> MAVFADLDLRAGSDLKALRGLVETAAHLGYSVVAINHIVDFKEKKQEIEKPVAVSELFTTLPIVQGKSRPIKILTRLTIIVSDPSHCNVLRATSSRARLYDVVAVFPKTEKLFHIACTHLDVDLVCITVTEKLPFYFKRPPINVAIDRGLAFELVYSPAIKDSTMRRYTISSALNLMQICKGKNVIISSAAERPLEIRGPY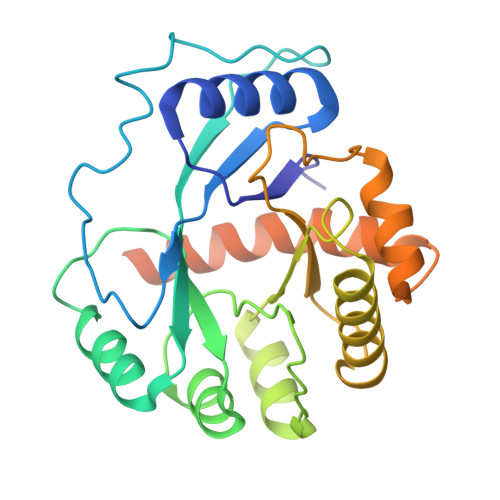DVANLGLLFGLSESDAKAAVSTNCRAALLHGETRKTAFGIISTVKKPRPSEGDEDCLPASKKAKCEG> APPSVFAEVPQAQPVLVFKLTADFREDPDPRKVNLGVGAYRTDDCHPWVLPVVKKVEQKIANDNSLNHEYLPILGLAEFRSCASRLALGDDSPALKEKRVGGVQSLGGTGALRIGADFLARWYNGTNNKNTPVYVSSPTWENHNAVFSAAGFKDIRSYRYWDAEKRGLDLQGFLNDLENAPEF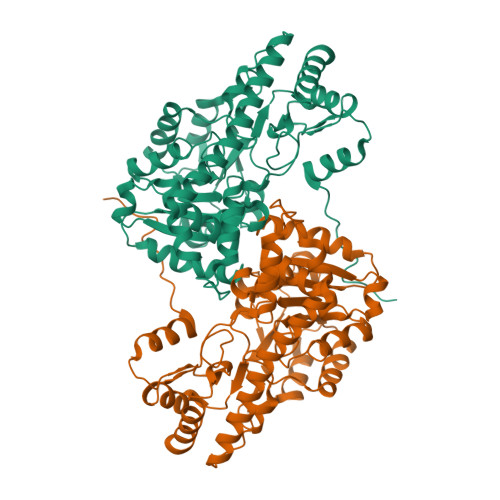SIVVLHACAHNPTGIDPTPEQWKQIASVMKHRFLFPFFDSAYQGFASGNLERDAWAIRYFVSEGFEFFCAQSFSKNFGLYNERVGNLTVVGKEPESILQVLSQMEKIVRITWSNPPAQGARIVASTLSNPELFEEWTGNVKTMADRILTMRSELRARLEALKTPGTWNHITDQIGMFSFTGLNPKQVEYLVNEKHIYLLPSGRINVSGLTTKNLDYVATSIHEAVTKIQ>LQHQNPQQLSSNLWAAVRARGCQFLGPAMQEEALKLVLLALEDGSALSRKVLVLFVVQRLEPRFPQASKTSIGHVVQLLYRASCFKVTKRDEDSSLMQLKEEFRTYEALRREHDSQIVQIAMEAGLRIAPDQWSSLLYGDQSHKSHMQSIIDKLQTPASFAQSVQELTIALQRTGDPANLNRLRPHLELL[4x]

The Roquin protein is essential in T cells for the prevention of autoimmune disease. We have recently reported structural and functional data of the Roquin-1 ROQ domain bound to a canonical constitutive decay element (CDE), a short stem loop (SL) that acts as a cis-regulatory RNA element in the 3′-untranslated regions (3′-UTRs) of target genes such as Tnf. The ROQ domain adopts an extended winged helix fold that engages predominantly non-sequence-specific protein–RNA contacts and mainly recognizes the shape of the canonical Tnf CDE RNA. Here we present structural and functional evidence for a greatly expanded repertoire of RNA elements that are regulated by Roquin as demonstrated with a novel U-rich hexaloop SL in the 3′-UTR of Ox40 bound to the Roquin-1 ROQ domain.

We set out to identify Roquin-bound RNA motifs in an unbiased manner by performing SELEX experiments. Evaluation of the structural context for the SELEX-derived motif suggested a putative SL formation with six unpaired nucleotides in a loop followed by a 5–8 nt stem, with one base in the stem not being paired. The structures of ROQ bound to the 20-mer ADE SL and to the 22-mer Ox40 ADE-like SL RNAs were refined to a resolution of 3.0 and 2.2 Å, respectively. In both structures the RNA adopts an SL fold, where the hexaloop is located in the vicinity of the carboxy-terminal end of ROQ helix α4 and the N-terminal part of β3. Interestingly, although the sequences of the ADE SL and ADE-like SL RNAs are different, the overall structures and protein–RNA contacts are virtually identical. The only differences are a C19 bulge, the non-Watson–Crick G6–G15 base pair and the interaction of U1 with Trp184 and Phe194 in the ADE-like SL RNA. Notably, we also found an unambiguous imino proton signal for G15, but not G6, in the ADE SL, indicating a non-Watson–Crick G–G base pair at this position. On the other hand, comparison of ROQ domain binding with the ADE and with the ADE-like SL RNAs indicates almost identical NMR spectra and CSPs. In summary, similar to the CDE SL, both the ADE SL and ADE-like SL RNAs are recognized mainly by non-sequence-specific contacts. In this respect, it is interesting to note that symmetry-related RNA molecules of both Tnf CDE and ADE SL RNAs are found in the respective crystal lattice in a position that corresponds to the recognition of dsRNA in the B site111222.>[14x]MAQNDNYIYSTEVGGVGGTPFTFMQES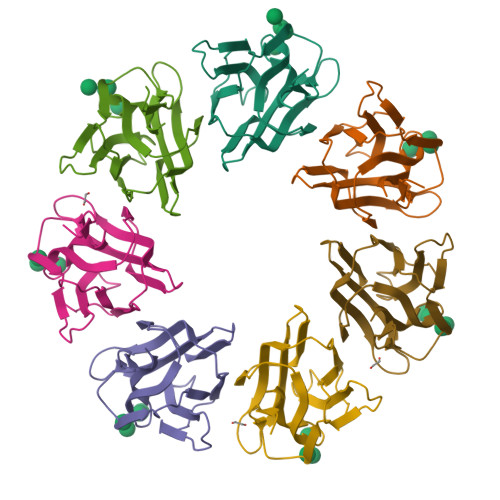GTITSIKFNWSDQYKLLHHIEVKFINNANIYATGDPKGNHEVILEIDDDETIIGSVIGYKKGNDGRCTGVKLTTSKGKSIMAGYFEESLITTYTGKLAGIKGGAGSDIDRLGLIFLKK> MAYTRSKIVDLVDGKIDPDTLHQMLSTPKDPERFVTYVEILQERMPWDDKIILPLGPKLFIVQQKVSKKWTVRCECGHDFCDWKDNWKLHARVHVRDTPQKMEEIYPRLMAP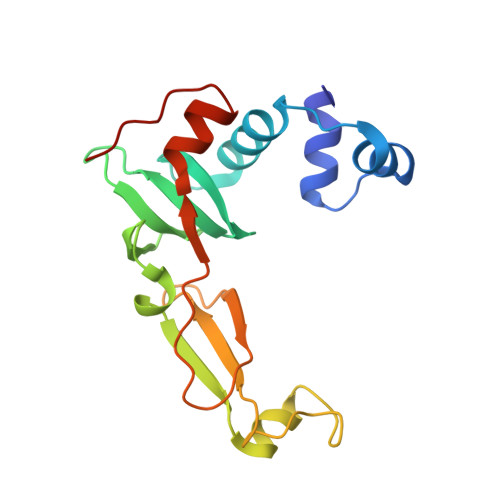TPSWQVIREYFCPECGTLHDVEAPTPWYPVIHDFSPDIEGFYQEWLGLPVPERADA> GRQNLYFQGMPKVIIFTDFDGTVTGKSGNETVFTEFYQSLLQGYKKDVEQDYKNTPMKDPIEAQALFEAKYGKYNENFDHDQQDVDFLMSPEAVAFFHEVLKNDDVTVNIVTKNRAEYIKAVFKYQGFSDEEISKLTILESGYKFNDVNSRLNHPTERANRVYILDDSPTDYAEMLRAVK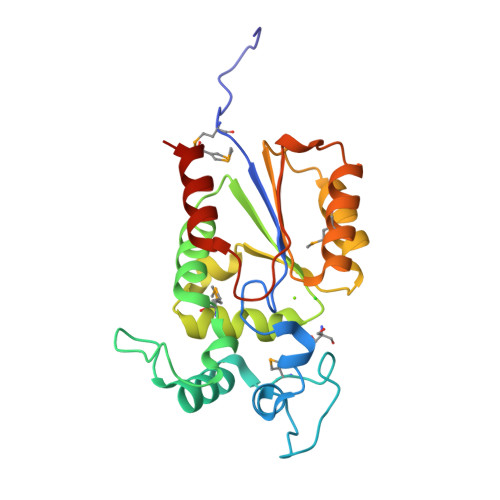GKGYNEEEIRGYRKNPGEFEWSQYLEDVREMFPPKEN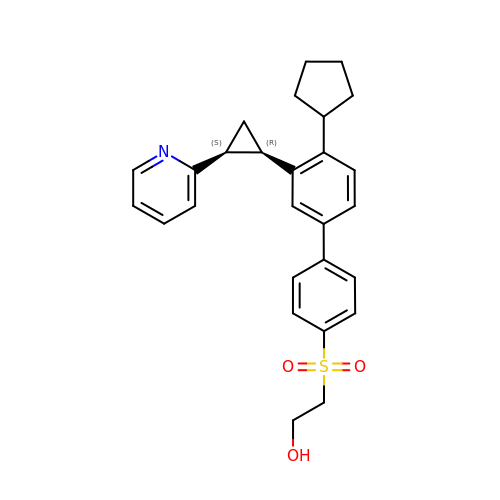2-[4-[4-cyclopentyl-3-[(1~{R},2~{S})-2-pyridin-2-ylcyclopropyl]phenyl]phenyl]sulfonylethanol | C27 H29 N O3 S | SQNBJZZENOHHKX-UIOOFZCWSA-N>[6x]AQQMPSLAPMLEKVMPSVVSINVEGSTTVNT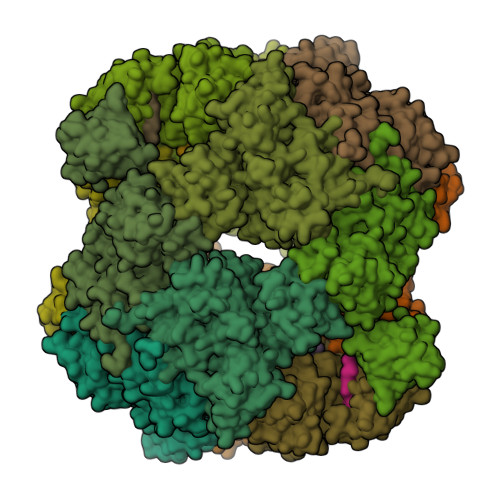PRMPRNFQQFFGDDSPFCQEGSPFQSSPFCQGGQGGNGGGQQQKFMALGSGVIIDADKGYVVTNNHVVDNATVIKVQLSDGRKFDAKMVGKDPRSDIALIQIQNPKNLTAIKMADSDALRVGDYTVAIGNPFGLGETVTSGIVSALGRSGLNAENYENFIQTDAAINRGNAGGALVNLNGELIGINTAILAPDGGNIGIGFAIPSNMVKNLTSQMVEYGQVKRGELGIMGTELNSELAKAMKVDAQRGAFVSQVLPNSSAAKAGIKAGDVITSLNGKPISSFAALRAQVGTMPVGSKLTLGLLRDGKQVNVNLELQQSSQNQVDSSSIFNGIEGAEMSNKGKDQGVVVNNVKTGTPAAQIGLKKGDVIIGANQQAVKNIAELRKVLDSKPSVLALNIQRGDSTIYLLMQ;>CYYKI[12x]(1S,5S,6R)-10-(benzo[d]thiazol-6-ylsulfonyl)-5-(methoxymethyl)-3-(pyridin-2-ylethyl)-3,10-diazabicyclo[4.3.1]decan-2-one 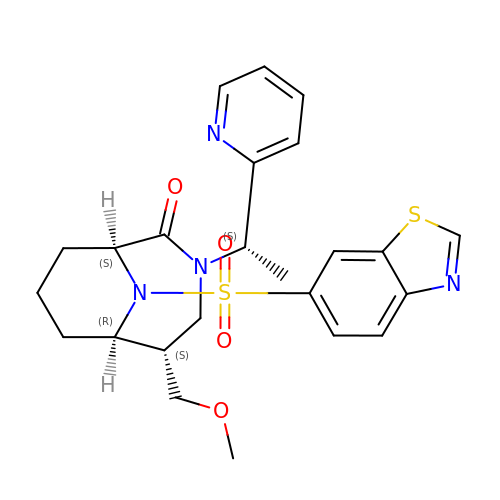| C24 H28 N4 O4 S2 | KWBWMGZANKQLDI-DVRVPYBTSA-N>MMSYQPQTEAATSRFLNVEEAGKTLRIHFNDCGQGDETVVLLHGSGPGATGWANFSRNIDPLVEAGYRVILLDCPGWGKSDSVVNSGSRSDLNARILKSVVDQLDIAKIHLLGNSMGGHSSVAFTLKWPERVGKLVLMGGGTGGMSLFTPMPTEGIKRLNQLYRQPTIENLKLMMDIFVFDTSDLTDALFEARLNNMLSRRDHLENFVKSLEANPKQFPDFGPRLAEIKAQTLIVWGRNDRFVPMDAGLRLLSGIAG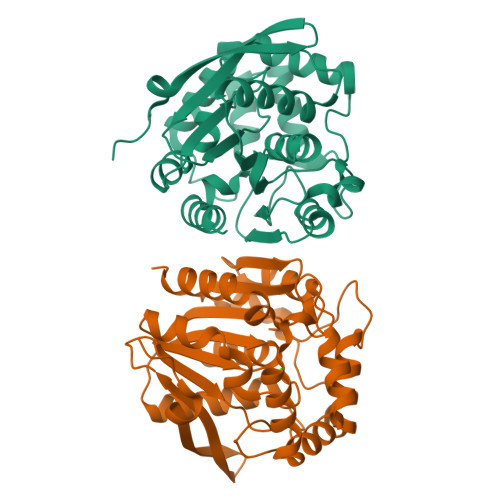SELHIFRDCGHWAQWEHADAFNQLVLNFLARP[4x]> MELQQNFTDNNSIKYTAILILIAFAFSVLARLYWVAWASEFYEFFFNDQLMITTNDG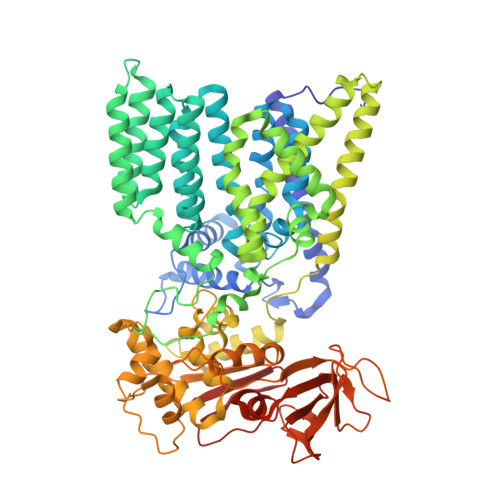YAFAEGARDMIAGFHQPNDLSYFGSSLSTLTYWLYSILPFSFESIILYMSTFFASLIVVPIILIAREYKLTTYGFIAALLGSIANSYYNRTMSGYYDTDMLVLVLPMLILLTFIRLTINKDIFTLLLSPVFIMIYLWWYPSSYSLNFAMIGLFGLYTLVFHRKEKIFYLTIALMIIALSMLAWQYKLALIVLLFAIFAFKEEKINFYMIWALIFISILILHLSGGLDPVLYQLKFYVFKASDVQNLKDAAFMYFNVNETIMEVNTIDPEVFMQRISSSVLVFILSFIGFILLLKDHKSMLLALPMLALGFMALRAGLRFTIYAVPVMALGFGYFLYAFFNFLEKKQIKLSLRNKNILLILIAFFSISPALMHIYYYKSSTVFTSYEASILNDLKNKAQREDYVVAWWDYGYPIRYYSDVKTLIDGGKHLGKDNFFSSFVLSKEQIPAANMARLSVEYTEKSFKENYPDVLKAMVKDYQKTSAKDFLESLNDPNFKIDTPKTRDVYIYMPYRMLRIMPVVAQFANTNPDNGEQEKSLFFSQANPLDQDKKQGSITLDNGVEISNDYRSLKIEGNSIPLKAFVDIESITNGKFYYNEIDSKAQIYLLYLREYKSYVILDESLYNSSYIQMFLLNQYDQDLFEQITNDTRAKIYRLKREFHHHHHHHHHH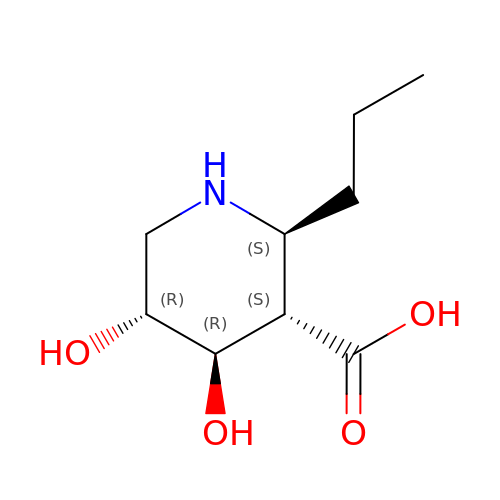(2~{S},3~{S},4~{R},5~{R})-4,5-bis(oxidanyl)-2-propyl-piperidine-3-carboxylic acid | C9 H17 N O4 | FBBVTGIVZAYALR-YWIQKCBGSA-N> MRPYTLSVALPGSILDNAQSPELRTYLAGQIARACAIFCVDEIVVFDEEGQDAKTVEGEFTGVGKKGQAC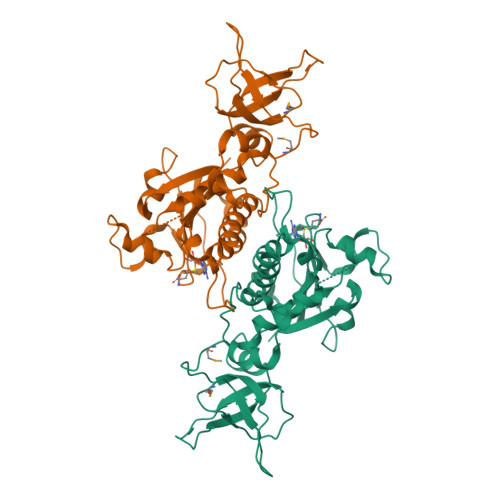VQLARILQYLECPQYLRKAFFPKHQDLQFAGLLNPLDSPHHMRQDEESEFREGIVVDRPTRPGHGSFVNCGMKKEVKIDKNLEPGLRVTVRLNQQQHPDCKTYHGKVVSSQDPRTKAGLYWGYTVRLASCLSAVFAEAPFQDGYDLTIGTSERGSDVASAQLPNFRHALVVFGGLQGLEAGADADPNLEVAEPSVLFDLYVNTCPGQGSRTIRTEEAILISLAALQPGLIQAGARHT~{N}-[4-(3-hydroxyphenyl)-1,3-thiazol-2-yl]-2-[4-oxidanylidene-3-(2-phenylethyl)pteridin-2-yl]sulfanyl-ethanamide | C25 H20 N6 O3 S2 | 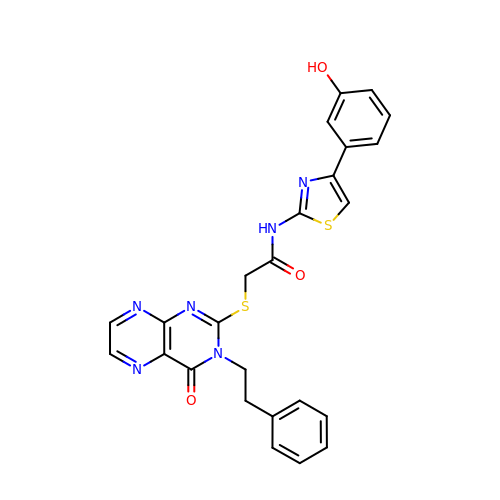KPWZZHNCABTUGN-UHFFFAOYSA-N> MASFKSIAALIALIFAVNAAQIGPVTDLHITNANISPDGFSRPAVLAGGTFPGPTIAGNTGDNFQITVFNDLTDPSMLTDTSIHWHGLFQKGTNWADGPAFVTQCPIITGQSFDYNFNVPGQAGTFWYHSHLSTQYCDGLRGPFVVYDPNDPNASLYDVDDDTTIITLADWYHTLAQQEPIGAAITADATLINGLGRSFTNTTASPLSVITVQSGKRYRMRLVSISCDPNYLFSIDGHDMTIIEVDGVNSQQLTVDQIQIFAAQRYSFVL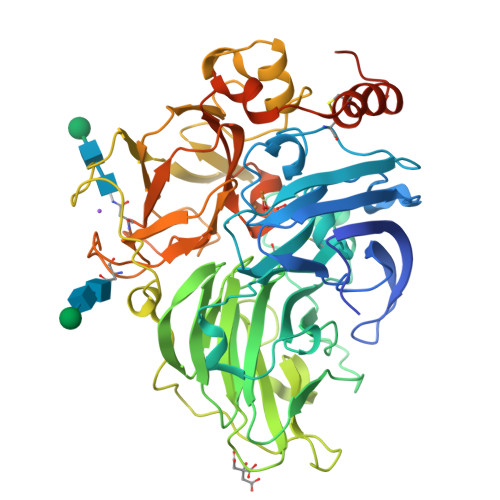NANQPVGNYWIRAQPNSGGQGFDGGINSAILRYEGATVEDPTTTAPTTFSNPLVETDLHPLADLGVPGQPFRGGADDPLVLNLAFANGRFSIDGVSFVPPTVPVLLQILSGAQNAQDLLPAGSVISLPSNSVIEVALPAGAAGGPHPFHLHGHNFAVVQSANNATPNYVNPIWRDTVSIGGTGDNVTIRFTTNNPGPWFLHCHIDWHLEAGFAIVFAEDIPDTASANPVPQAWSDLCPAYDQAHNISTATRQDFQILCICGILHVNFRQEERCGIS> TT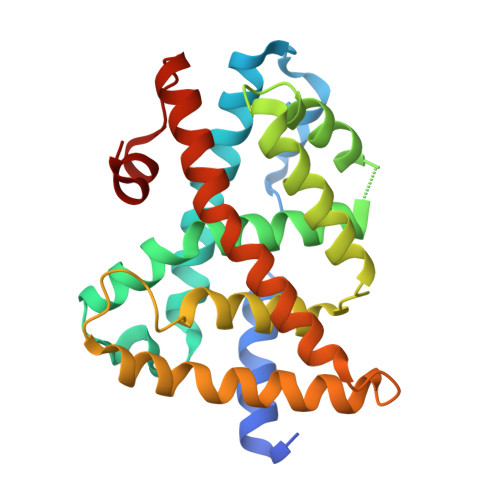KSCREKTELTPDQQTLLHFIMDSYNKQRMPQEITNKILKEEFSAEENFLILTEMATNHVQVLVEFTKKLPGFQTLDHEDQIALLKGSAVEAMFLRSAEIFNKKLPSGHSDLLEERIRNSGISDEYITPMFSFYKSIGELKMTQEEYALLTAIVILSPDRQYIKDREAVEKLQEPLLDVLQKLCKIHQPENPQHFACLLGRLTELRTFNHHHAEMLMSWRVNDHKFTPLLCEIWDVQ>[2x]MKSCAILAALGCLAGSVLGHGQVQNFTINGQYNQGFILDYYYQKQNTGHFPNVAGWYAEDLDLGFISPDQYTTPDIVCH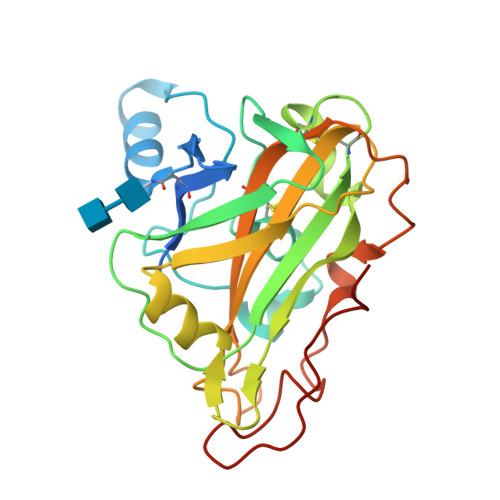KNAAPGAISATAAAGSNIVFQWGPGVWPHPYGPIVTYVVECSGSCTTVNKNNLRWVKIQEAGINYNTQVWAQQDLINQGNKWTVKIPSSLRPGNYVFRHELLAAHGASSANGMQNYPQCVNIAVTGSGTKALPAGTPATQLYKPTDPGILFNPYTTITSYTIPGPALWQG> MGSSHHHHHHSAGENLYFQGTLPRETDEEPEEPGRRGSFVEMVDNLRGKSGQGYYVEMTVGSPPQTLNILVDTGSSNFAVGAAPHPFLHRYYQRQLSSTYRDLRKGVYVPYTQGKWEGELGTDLVSIPHGPNVTVRANIAAITESDKFFINGSNWEGILGLAYAEIARPDDSLEPFFDSLVKQTHVPNLFSLQLCGAGFPLNQSEVLASVGGSMIIGGIDHSLYTGSLWYTPIRREWYYEVIIVRVEINGQDLKMDCKEYNYDKSIVDSGTTNLRLPKKVFEAAVKSIKAASSTEKFPDGFWLGEQLVCWQAGTTPWNIFPVISLYLMGEVTNQSFRITILPQQYLRPVEDVATSQDDCY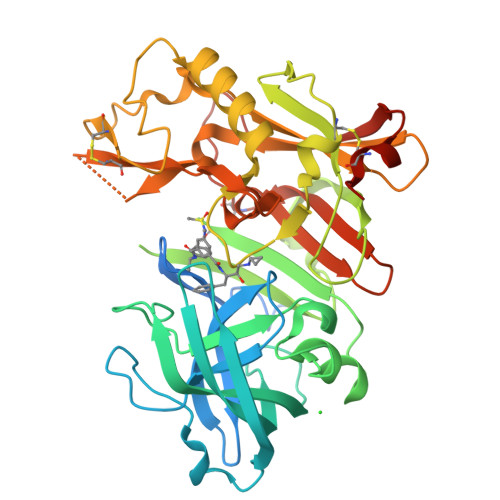KFAISQSSTGTVMGAVIMEGFYVVFDRARKRIGFAVSACHVHDEFRTAAVEGPFVTLDMEDCGYNIPQTDEST>[2x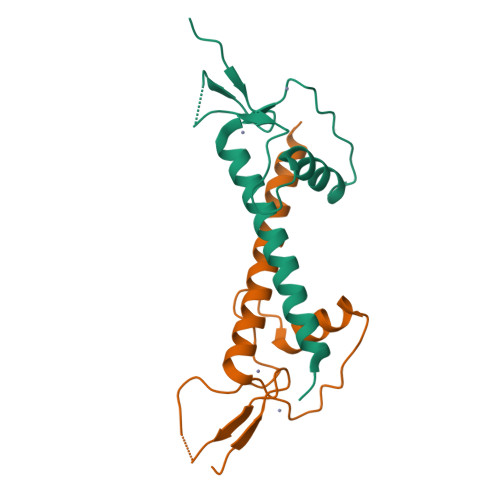]PEFMDTCFFCGAVDLSDTGSSSSMRYETLSAKVPSSQKTVSLVLTHLANCIQTQLDLKPGARLCPRCFQELSDYDTIMVNLMTTQKRLTTQLKLDK>[2x]MATLTAKNLAKAYKGRRVVEDVSLTVNSGEIVGLLGPNGAGKTTTFYMVVGIVPRDAGNIIIDDDDISLLPLHARARRGIGYLPQEASIFRRLSVYDNLMAVLQIRDDLSAEQREDRANELMEEFHIEHLRDSMGQSLSGGERRRVEIARALAANPKFILLDEPFAGVDPISVIDIKRIIEHLRDSGLGVLITDHNVRETLAVCERAYIVSQGHLIAHGTPTEILQDEHVKRVYLGEDFRL;> MSKARRWVIIVLSLAVLVMIGINMAEKDDTAQVVVNNNDPTYKSEHTDTLVYNPEGALSYRLIAQHVEYYSDQAVSWFTQPVLTTFDKDKIPTWSVKADKAKLTNDRMLYLYGHVEVNALVPDSQLRRITTDNAQINLVTQDVTSEDLVTLYGTTFNSSGLKMRGNLRSKNAELIEKVRTSYEIQNKQTQP;> MIIIRYLVRETLKSQLAILFILLLIFFCQKLVRILGAAVDGDIPANLVLSLLGLGVPEMAQLILPLSLFLGLLMTLGKLYTESEITVMHACGLSKAVLVKAAMILAVFTAIVAAVNVMWAGPWSSRHQDEVLAEAKANPGMAALAQGQFQQATNGSSVLFIESVDGSDFKDVFLAQIRPKGNARPSVVVADSGHLTQLRDGSQVVTLNQGTRFEGTALLRDFRITDFQDYQAIIGHQAVALDPNDTDQMDMRTLWNTDTDRARAELNWRITLVVTVFMMALMVVPLSVVNPRQGRVLSMLPAMLLYLLFFLIQTSLKSNGGKGKLDPTLWMWTVNLIYLALAIVLNLWDTVPVRRLRASFSRKGAV;> MQPFGVLDRYIGKTIFTTIMMTLFMLVSLSGIIKFVDQLKKAGQGSYDALGAGMYTLLSVPKDVQIFFPMAALLGALLGLGMLAQRSELVVMQASGFTRMQVALSVMKTAIPLVLLTMAIGEWVAPQGEQMARNYRAQAMYGGSLLSTQQGLWAKDGNNFVYIERVKGDEVLGGISI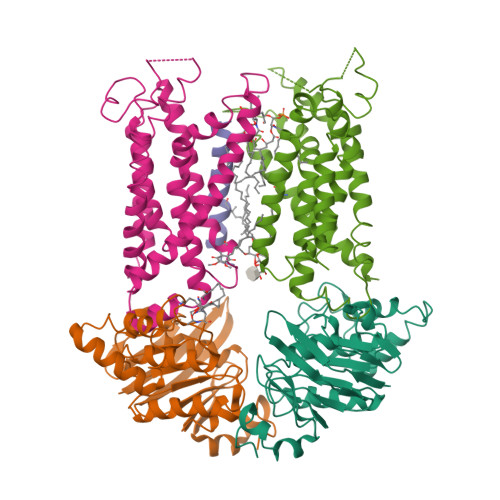YAFNENRRLQSVRYAATAKFDPEHKVWRLSQVDESDLTNPKQITGSQTVSGTWKTDLTPDKLGVVALDPDALSISGLHNYVKYLKSSGQDAGRYQLNMWSKIFQPLSVAVMMLMALSFIFGPLRSVPMGVRVVTGISFGFVFYVLDQIFGPLTLVYGIPPIIGALLPSASFFLISLWLLMRKS> MSVETPSALADSSPHTAPGSAGRSLELGAADIQDLESFEAGRGALPARAYLQSDAPRLSLNGEWQFRLSPGSRVAPDDGWQLGEALNGFESLPVPSSWPMHGHGAPAYTNVQFPFAVEPPHVPEANPIGDHLVVFEAGPEFFPHALLRFDGIESAGTVWLNGVELGTTRGSRLAHEFDVSGILEQGENTLAVRVAQFSAASYVEDQDMWWLPGIFRDVTLQARPAAGIDDVFVHAGYDHITGEGILKVEASRGGQAIDAVVRVPELALELAAGTEVRVPAVEPWSAEVPKLYEAAVSAAGESVALQIGFRSIAIEDAQFKVNGRRILLRGVNRHEHHPRLGRVVPRDVVEAELRLMKQHNINAIRTSHYPPHPQFLALADQLGFYVVLECDLETHGFESAGWAQNPSDDPQWEDALVDRMRRTVERDKNHASVVMWSLGNEAGTGRNLAAMSRWTKDRDPSRPIHYEGDWSSEHVDVYSRMYASQAETALIGQGIEPALNDAALDARRRAMPFVLCEYVHAMGNGPGGMSEYQALFEKYPRLMGGFVWEWLEHGITVSTADGVDHYGYGGDFGEEVHDGNFVTDGLVDADRRPRPGLLDFKKVIEPLRIDVARDWTGFTLRNGQDFADTSAFSFRYEVEADGGALDGGTVDVAPVAPQSETVVELPGSVAALAAGLSDGRPAVLTVRAVLGADSAWADAGHEVAWGQSVREPGAPVPPAPVEPVQVQDSELTLGPVVFSRATGMPTSIGGVPVEKLGLTLWWAPTDNDLGREWGGADERPLATQWKD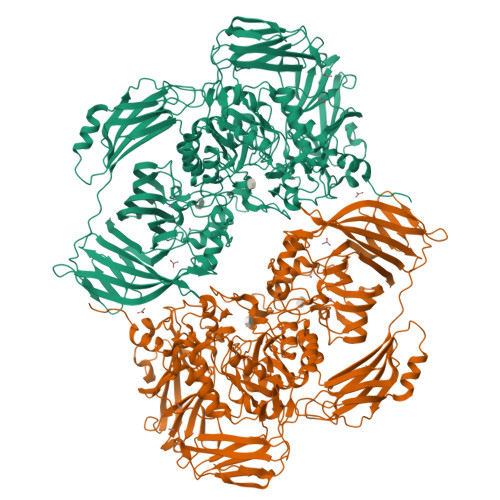AGLNRLHTRLLGISANPGQDGGETLTVRTRVSAADKQYGVLVDYTWSTDGETVGLRTQVRRDGTWVNRGFEVEWARIGLEFVLGEETELVSWFGQGPHQSYPDTGQGARAGWFSLPLAKMDVEYVRPQECGARSGSRSAALQLGGRTLEICGDPFALTVRPYSQDVLDAAAHRPDLKADGRTYLYVDHALRGVGTAACGPGVLEQYRLKPRDADFILTLKVRS>[2x]MAHHHHHHGHTPRQPTDSPLYPLLSAAAEFYKQALKSHPARKAAVNYLKGRGLTGEIARDFGLGFAPPGWDNLLKHLGGDNLQLKA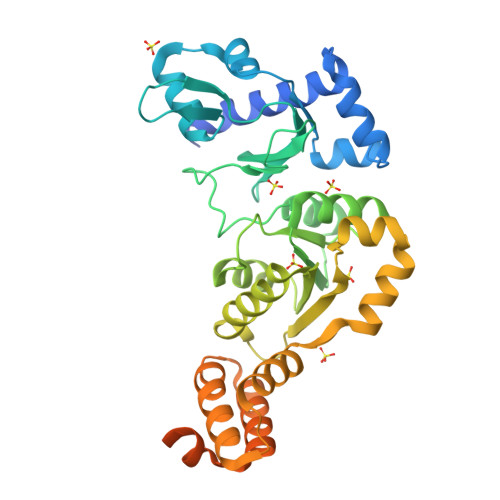MLDAGLLVENSDTGKRYDRFRDRVMFPIRDSRGRIIAFGGRVLGDDKPKYLNSPETPVFHKGQELYGLYEARQKNRDLDEIMVVEGYMDVIALAQQGIRNAVATLGTATSEEHIKRLFRLVPSILFCFDGDQAGRKAAWRALESVLPNLQDGKRVRFLFLPEGEDPDSLVRAEGEDAFRARITQQAQPLAEYFFQQLMLEADPATLEGKAHLATLAAPLLEKIPGNNLRLLMRQRLSEITGLSGENIGQLAHHSPPPSSMDHGASGVLDGDDYFAASAYYENEPSHAPFDAAPGYVEAQPRKS> GEADMDFLRNLFSQTLSLGSQKERLLDELTLEGVARYMQSERCRRVICLVGAGISTSAGIPDFRSPSTGLYDNLEKYHLPYPEAIFEISYFKKHPEPFFALAKELYPGQFKPTICHYFMRLLKDKGLLLRCYTQNIDTLERIAGLEQEDLVEAHGTFYTSHCVSASCRHEYPLSWMKEKIFSEVTPKCEDCQSLVKPDIVFFGESLPARFFSCMQSDFLKVDLLLVMGTSLQVQPFASLISKAPLSTPRLLINKEKAGQSDPFLGMIMGLGGGMDFDSKKAYRDVAWLGECDQGCLALAELLGWKKELEDLVRREHASIDAQS;> KGLGKGGAKRHRK

Human sirtuin isoform 2 (SIRT2) is an NAD+-dependent enzyme that functions as a lysine deacetylase and defatty-acylase. By catalyzing the removal of protein acyl modifications, SIRT2 regulates diverse processes including cancer growth, neurodegeneration, metabolism, and inflammation. The acyl substrates of SIRT2 are chemically diverse and range from small modifications such as acetyl-lysine to much larger, fatty modifications such as myristoyl-lysine. Here, we report that SIRT2 readily dimerizes in solution and in cells and that dimerization affects its ability to remove different acyl modifications from substrates. In this work, we report our observations that SIRT2 does indeed oligomerize in solution, favoring a homodimer at concentrations greater than ∼100 nM.

The experiments above strongly indicated that the interaction of SIRT2cat with the myristoyl modification on the H4K16 peptide was essential for driving the dimer to monomer transition. To better visualize this, we cross-linked SIRT2cat while bound to a fluorescein-labeled, myristoyl-H4K16 peptide called “FAM-myristoyl-H4K16”. This fluorescent myristoyl peptide also caused a SIRT2cat transition from dimer to monomer (lane 4). We also mixed SIRT2cat and FAM-myristoyl-H4K16 peptide at 52 μM each and analyzed their complex with SEC, which confirmed that the protein/peptide complex was monomeric. FAM-myristoyl-H4K16 peptide and the unlabeled myristoyl-H4K16 peptide had nearly identical affinity for SIRT2cat using a gel shift assay (Kd = 1–2 μM), and SIRT2cat processes FAM-myristoyl-H4K16 peptide as a conventional myristoyl substrate. Instead, we hypothesized that the position of interface residues should change between the structures of apo-SIRT2cat and myristoyl peptide-bound SIRT2cat if that interface was altered during substrate binding and was important for the dimer to monomer transition. Thus, we aligned our crystal structure of SIRT2cat bound to myristoyl peptide to each molecule of the apo-SIRT2cat trimer to observe structural differences at Interface 1 or Interface 2. The backbone atoms near Interface 1 overlapped perfectly in the aligned structures and did not change their position when SIRT2cat was substrate-bound. On the other hand, the C-terminal helix at Interface 2 tilted inward 4° on its hinge when the protein was bound to myristoyl peptide, suggesting Interface 2 had a structural change that could affect protein dimerization. Five of the residues were on the SIRT2cat C-terminal helix, and the sixth residue we mutated (Q142) dramatically repositioned to contact the C-terminal helix in myristoyl peptide-bound SIRT2cat, but not apo-SIRT2cat.>[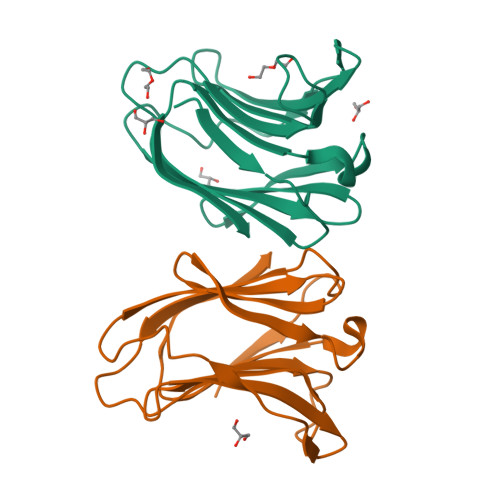2x]SNVPHKSSLPEGIAPGTVLRIRGLVPPNASRFHVNLLCGEEQGSDAALHFNPRLDTSEVVFNSKEQGSWGREERGPGVPFQRGQPFEVLIIASDDGFKAVVGDAQYHHFRHRLPLARVRLVEVGGDVQLDSVRIF>MANCERTFIAIKPDGVQRGLVGEIIKRFEQKGFRLVGLKFMQASEDLLKEHYVDLKDRPFFAGLVKYMHSGPVVAMVWEGLNVVKT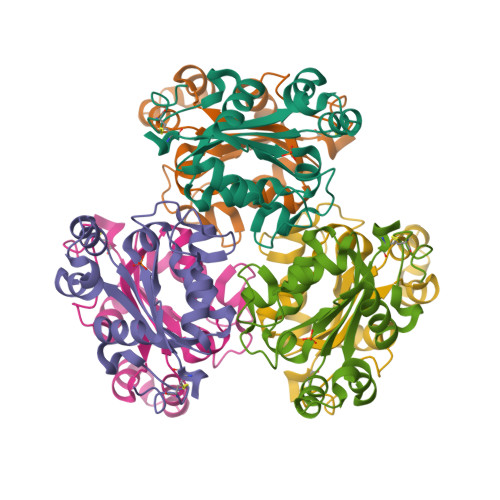GRVMLGETNPADSKPGTIRGDFCIQVGRNIIHGSDSVESAEKEIGLWFHPEELVDYTSCAQNWIYE[2x]Contactins (CNTNs) are neural cell adhesion molecules that encode axon-target specificity during the patterning of the vertebrate visual and olfactory systems. Because CNTNs are tethered to the plasma membrane by a glycosylphosphatidylinositol anchor, they lack an intracellular region to communicate across the membrane. Instead, they form coreceptor complexes with distinct transmembrane proteins to transmit signals inside the cell. Finally, structural analyses of five CNTN–amyloid pairs indicate that these proteins interact through a conserved interface involving the second fibronectin type III repeat of CNTNs and the copper-binding domain of amyloid proteins.

In addition, complexes formed by chicken CNTN3(FN1–FN3) and APP(E1) also proved recalcitrant to crystallization. To resolve this issue, we designed a fusion protein of CNTN3 and APP, speculating that it might yield suitable crystals. We thus fused chicken CNTN3 to APP by inserting a GGGSGGGS linker between the C terminus of the FN2 repeat of CNTN3 and the N terminus of the E1 domain of chicken APP. This chimeric protein crystallized readily, and we refined the structure of the CNTN3–APP fusion to 2.75 Å (Rwork/Rfree = 0.197/0.231). Overall, the binding sites identified in the structures of the CNTN5–APP complex and the CNTN3–APP fusion protein are similar to the one identified in CNTN4–APP structure. Residue H137 in APP contacts Y681 in CNTN3 (Y853 in CNTN5), and its side chain forms a hydrogen bond with the carboxylate group of E686 (D858 in CNTN5). H137 also packs against V652 in CNTN3, as is observed at the CNTN4–APP interface. In the CNTN3–APP structure, we observed a hydrogen bond between the hydroxyl group of Y681, which hydrogen bonds with E139. At the CNTN3–APP interface, residue T651 forms a hydrogen bond with S124. This contact is identical to the T751–S124 hydrogen bond observed in the CNTN4–APP complex.

>[2x]GPGSPGPPEHVRVDEITDTTAQISWQEGTDNHSPVTAYTIQARTPFSVGWQRVTTVPDVIDGNTFTTTVVDLNPWVEYEFRVVASNKIGGGEPSLPSEKVRTEEAVPEIPPAEVSGGGGSRSELVITWDPIPEELQNGEGFGYVVAFRPFGTTTWIQTVVTSPDTPRYVFRNESILPFSPYEVKVGVYNNKGEGPFSSITTVFSAEGGGSGGGSEVPADGNAGLLAEPQIAMFCGKLNMHMNVQNGKWESDPSGTKTCIDTKEGILQYCQEVYPELQITNVVEANQPVTIQNWCKRGWKQCNGHPHIVVPYRCLVGEFVSDALLVPDKCKLLHQERMDVCETHLHWHTVAKESCSEKSMNLHDYGMLLPCGIDKFRGVEFVCCPLAEESDNLDSAAA>[2x]MEYEWKPDEQGLQQILQLLKESQSPDTTIQRTVQQKLEQLNQYPDFNNYLIFVLTKLKSEDEPTRSLSGLILKNNVKAHFQNFPNGVTDFIKSECLNNIGDSSPLIRATVGILITTIASKGELQNWPDLLPKLCSLLDSEDYNTCEGAFGALQKICEDSAEILDSDVLDRPLNIMIPKFLQFFKHSSPKIRSHAVACVNQFIISRTQALMLHIDSFIENLFALAGDEEPEVRKNVCRALVMLLEVRMDRLLPHMHNIVEYMLQRTQDQDENVALEACEFWLTLAEQPICKDVLVRHLPKLIPVLVNGMKYSDIDIILLKGDVEEDETIPDSEQDIGGSGGSGDTISDWNLRKCSAAALDVLANVYRDELLPHILPLLKELLFHHEWVVKESGILVLGAIAEGCMQGMIPYLPELIPHLIQCLSDKKALVRSITCWTLSRYAHWVVSQPPDTYL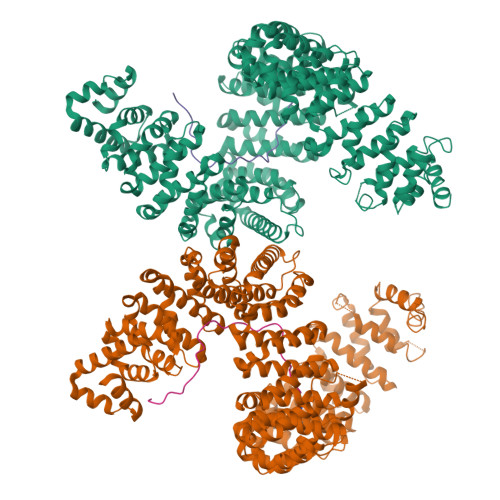KPLMTELLKRILDSNKRVQEAACSAFATLEEEACTELVPYLAYILDTLVFAFSKYQHKNLLILYDAIGTLADSVGHHLNKPEYIQMLMPPLIQKWNMLKDEDKDLFPLLECLSSVATALQSGFLPYCEPVYQRCVNLVQKTLAQAMLNNAQPDQYEAPDKDFMIVALDLLSGLAEGLGGNIEQLVARSNILTLMYQCMQDKMPEVRQSSFALLGDLTKACFQHVKPCIADFMPILGTNLNPEFISVCNNATWAIGEISIQMGIEMQPYIPMVLHQLVEIINRPNTPKTLLENTAITIGRLGYVCPQEVAPMLQQFIRPWCTSLRNIRDNEEKDSAFRGICTMISVNPSGVIQDFIFFCDAVASWINPKDDLRDMFCKILHGFKNQVGDENWRRFSDQFPLPLKERLAAFYGV;>GGSYNDFGNYNNQSSNFGPMKGGNFGGRSSGPYGGGGQYFAKPRNQGGY[2x]> GSEDFTFDGTKRLSVNYVKGILQPTDTCDIWDKIWNFQAKPDDLLISTYPKAGTTWTQEIVELIQNEGDVEKSKRAPTHQRFPFLEMKIPSLGSGLEQAHAMPSPRILKTHLPFHLLPPSLLEKNCKIIYVARNPKDNMVSYYHFQRMNKALPAPGTWEEYFETFLAGKVCWGSWHEHVKGWWEAKDKHRILYLFYEDMKKNPKHEIQKLAEFIGKKLDDKVLDKIVHYTSFDVMKQNPMANYSSIPAEIMDHSISPFMRKGAVGDWKKHFTVAQNERFDEDYKKKMTDTRLTFHFQF

Cytosolic sulfotransferases (SULTs) comprise a family of enzymes that catalyze the transfer of a sulfonate group from 3′-phosphoadenosine 5′-phosphosulfate (PAPS) to an acceptor group of the substrate. In doing so, SULTs modulate the activities of a large array of small endogenous and foreign chemicals, including drugs, toxic compounds, steroid hormones, and neurotransmitters. As expected, all SULTs share the same basic fold: a central four-stranded parallel β-sheet surrounded by α-helices and three loops that are often disordered (dashed lines) in the absence of PAP and/or substrate. The crystal structures of SULT1C3 bound to PAP, apo SULT1C2, a ternary complex of SULT1C2 bound to PAP, and the environmental toxin, pentachlorophenol (PCP), and SULT4A1 were solved at 3.2, 2.0, 1.8, and 2.2 Å, respectively.

In some cases, partial stabilization can be attributed to molecular packing in the crystal, as in, for example, the stabilization of α14 (green) in apo SULT1C2. Helices α4, α5, and αı5, and loops α5-α6 and α15-α16 are ordered only in the ternary complex, but not in the apo SULT1C2 structure. The degree of disorder and the exact conformation of these loops vary considerably across the family, but in general, the presence of ligands (cofactor and/or substrate) is coupled with increased order, namely, the formation of helices α4-α5 (gold), and α14-α15 (green). Thus, SULT1B1 and 1C2 appear to be much more closely related in terms of structure and activity than their global sequences would indicate.MgtE is a widely distributed Mg2+ channel in both prokaryotes and eukaryotes. The bacterial MgtE channels are highly selective for Mg2+, and are involved in the maintenance of the intracellular Mg2+ concentration. The full-length structure in the presence of Mg2+ revealed that MgtE forms a homodimer, consisting of five transmembrane helices, one plug helix, and the cytosolic region composed of the N-terminal domain and the tandemly repeated CBS domains. A comparative analysis of the Mg2+-bound and Mg2+-free cytosolic domain structures, together with molecular dynamic simulations, revealed that Mg2+ binding to the cytosolic domain stabilizes the closed conformation of MgtE, suggesting a Mg2+ homeostasis mechanism in which the MgtE cytosolic domain acts as a Mg2+ sensor to regulate the Mg2+ influx.

To gain further insights into the ATP-dependent modulation of the channel gating in MgtE, we determined the crystal structure of the full-length MgtE in complex with ATP at 3.6 Å resolution. The overall structure represents the closed conformation of the channel, and is essentially identical to the previously reported full-length structure, with a root mean squared deviation (RMSD) value of 0.38 Å for all Cα atoms. The electron density for Mg2+ corresponds to the Mg2+-binding sites (Mg1–Mg7) in the previously reported full-length structure. Consistent with the previous structure, the electron density for Mg7 is relatively weak, possibly indicating the weak affinity of the Mg7 site for Mg2+. We also determine the crystal structures of the full-length and the cytosolic domain of MgtE in complex with ATP, which reveal that ATP is recognized by the CBS domain of MgtE. ATP molecules are located proximal to the subunit interface between the N domain in one subunit and the CBS domain in the neighboring subunit. The ATP molecule is exclusively recognized by the CBS domain. Accordingly, while ATP can bind to MgtE to modulate the channel gating, MgtE either lacks or has very low ATPase activity. This conclusion is also supported by the crystal structures of the MgtE–ATP complex, where the γ-phosphate group of ATP is clearly observed. With ATP bound to the cytosolic domain, MgtE closes when the intracellular Mg2+ concentration is above the physiological range (1–2 mM) b.

>MGSSHHHHHHSSGLGVLPGGPLHMEEKLAVSLQEALQEGDTRALREVLEEIHPQDLLALWDELKGEHRYVVLTLLPKAKAAEVLSHLSPEEQAEYLKTLPPWRLREILEELSLDDLADALQAVRKEDPAYFQRLKDLLDPRTRAEVEALARYEEDEAGGLMTPEYVAVREGMTVEEVLRFLRRAAPDAETIYYIYVVDEKGRLKGVLSLRDLIVADPRTRVAEIMNPKVVYVRTDTDQEEVARLMADYDFTVLPVVDEEGRLVGIVTVDDVLDVLEAEATEDIHKLGAVDVPDLVYSEAGPVALWLARVRWLVILILTGMVTSSILQGFESVLEAVTALAFYVPVLLGTGGNTGNQSATLIIRALATRDLDLRDWRRVFLKEMGVGLLLGLTLSFLLVGKVYWDGHPLLLPVVGVSLVLIVFFANLVGAMLPFLLRRLGVDPALVSNPLVATLSDVTGLLIYLSVARLLLEAV[2x]>[2x]MDWEERENPKRLVKTFAFPNF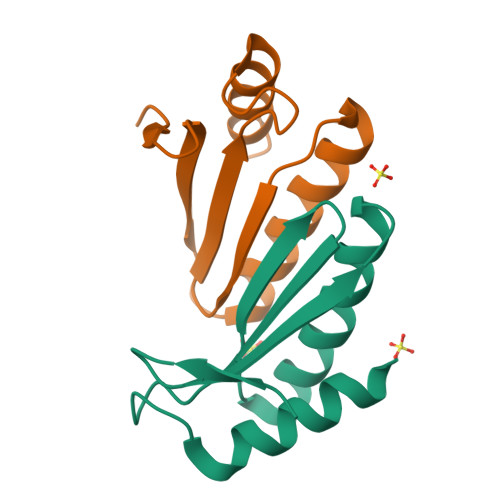REALDFANRVGALAERENHHPRLTVEWGRVTVEWWTHSAGGVTEKDREMARLTDALLQR>[2x]GNKIPTTMAFRTVTDVDNAVNGLYDLMSGSGYYGAAMFAYGDMKGDDMQSSEESGVCNTCY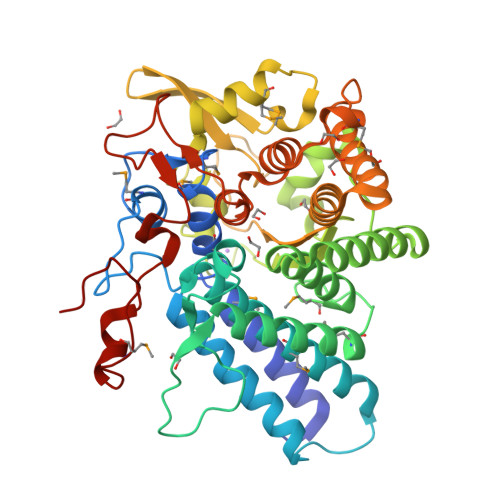MFNHRPNSLNAGSLWGRPFYILREAWNILNAIAEGKIESGDEKKLNALKGETMAVIALCQFDLTRCFGYPYTKDKGASLGAPLIDHLVGTYENPPRSTVAQAYDFIIETLEEAVTLMSEEKNNGRMNKYAARALLARIYLYHDDNRKAFDLADQLIKDADTSGSYALYPHEKYVAAWSVEAKFGSESFFEIANSVDDTPGRDSWGYLLNWYGYQKGFVTQKYAEQMLADPGDVRGHLLEENKYAGKTVWWLYKLRGTDLKTAPLECNNVVLRLSEVYLIAAEAGCKLGGDAAVQGLGYLNEIVKRGNPDNEVTMADYTLDRVLDERSKELVGEGHRFFDLLRNGKTIVRKGGYHLPSVDEEVDWDFYKCVLPIPEDQFIFSPEMEQNPGYPKN> WHDLKWPRDLRPLAHHDLLYMGQISEEDRGDFNATLRNFLVPRVVGSQKHREVREFIVRSLKDLDWDVEEDCFDGQTPHGIKPFCNVIATLNPSACHRLVLACHYDSLLHKEGTFIGATDSAVPCAQLLYLARSLNGKLQNQKTRGDGLTLQLVFFDGEEAFERWSSHDSLYGSRHLAQKWHEDRTSAERLESCLERSEIANQIDRMEVMVLLDLLGAENPRFYSYFGETQPVYRRLVNIESRLNDAGLMELPRRRRRTNYFSNSSTVGFIEDDHIPFLKRSVPIVHIIPSPFPDVWHTL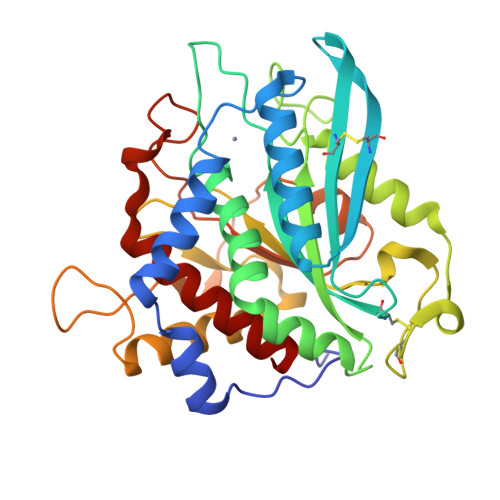DDNEQNLHHPTISNLNKIFKAFVSEYLQL> MAVPFVEDWDLVQTLGEGAYGEVQLAVNRVTEEAVAVKIVDMKRAVDCPENIKKEICINAMLNHENVVKFYGHRREGNIQYLFLEYCSGGELFDRIEPDIGMPEPDAQRFFHQLMAGVVYLHGIGITHRDIKPENLLLDERDNLKISDFGLATVFRYNNRERLLNKMCGTLPYVAPELLKRREFHAEPVDVWSCGIVLTAMLAGELPWDQPSDSCQEYSDWKEKKTYLNPWKKIDSAPLALLHKILVENPSARIT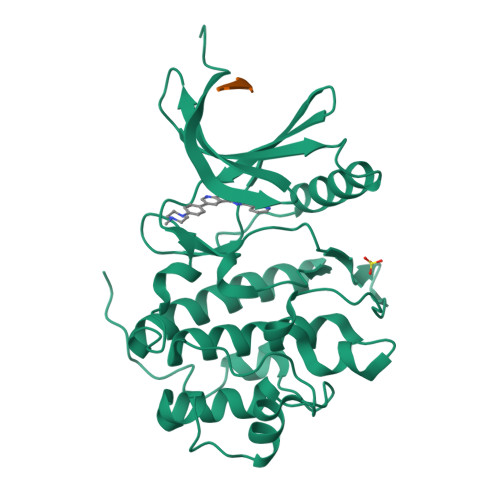IPDIKKDRWYNKPLKKGA;> ASVSA Rotaviruses are the leading etiologic agent of viral gastroenteritis in infants and young children worldwide and are responsible for an estimated 140,000 deaths each year in developing countries. Diverse interactions between histo-blood group antigens (HBGAs) and rotavirus have been described and it is believed that HBGAs expressed on the surface of target cells serve as viral receptors. The distal VP8* portion (~27 kDa, N-terminal) of the rotavirus spike protein VP4 from P, P, P and P genotypes recognize the secretor HBGAs. To understand the molecular basis of LNB and H1 recognition and binding to P VP8* we determined the crystal structure of the clinical isolate P[8]c VP8* in its apo form and bound to LNB and H1 glycans.

Crystals of P[8]c VP8* bound to H1 or its precursor LNB were obtained in a third different crystalline form and the structures of P[8]c VP8*-H1 and P[8]c VP8*-LNB complexes were solved to 1.8 and 1.3 Å, respectively. Two protomers of VP8* were present in the ASU of each of these crystals and, remarkably, only one out of the two protomers showed a bound glycan molecule. Sugar binding induces negligible conformational changes in the VP8* since the structural comparison of the glycan-bounded and glycan-free P[8]c VP8* protomers showed minimal differences (RMSD 0.22–0.35 Å). P[8]c VP8* binds H1 and LNB in a pocket formed by one of the β-sheets and the C-terminal α helix. Only seven residues recognize the LNB, contacting the N-acetyl-glucosamine moiety via L167, W174, T185, R209, and E212 and the galactose moiety via T184, T185, E212 and N216. The N-acetyl-glucosamine has a major contribution to the binding since it is inserted in the pocket while the galactose acquires a more superficial position. In this way, the N-acetyl-glucosamine ring is packet between W174 and R209 that define two faces of the binding site and the O4 and O6 oxygens mediated hydrogen-bonds with E212 that it placed at the bottom of the pocket. A close view of the relative disposition of the precursor LNB moiety in both P[8]c VP8* complexes after superimposition of VP8* proteins showed some differences but not so for the interacting residues. If, alternatively, the N-acetyl-glucosamine moieties from both structures are superimposed it becomes visible that the galactose moiety occupies a more solvent-exposed position in the LNB structure compared to H1, explaining its weaker binding in comparison with this antigen. The atomic resolution of the diffraction data and the high quality of the density maps derived from these data allows modeling accurately the ligand structures to observe these differences. This observation indicates that the L-fucose moiety induces an LNB conformation more suitable for the union to VP8*.

>GSMLDGPYQPTTFTPPSDYWILINSNTNGVVYESTNNSDFWTAVIAVEPHVDPVDRQYNVFGENKQFNVRNDSDKWKFLEMFRGSSQNDFYNRRTLTSNTRLVGILKYGGRIWTFHGETPRATTDSSNTANLNGISITIHSEFYIIPRSQESKCNEYINNGL[2x]> MIDLLQADGNALPSAVKLAYSPASKTFESYRVMTQVHTNDATKKVIVKLADTPQLTDVLNSTVQMPISVSWGGQVLSTTAKEFEAAALGYSASGVNGVSSSQELVISAAPKTAGTAPTAGNYSGVVSLVMTLGSDNKQVEKNITVTA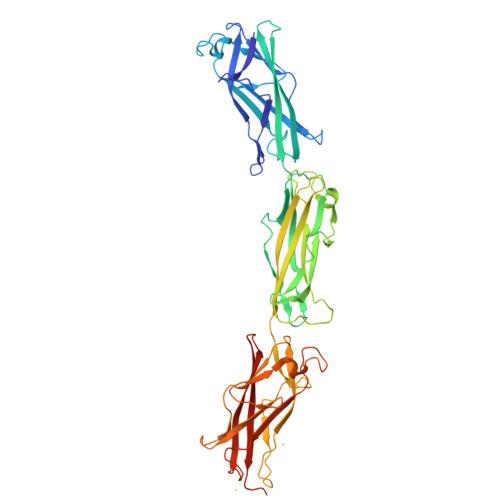SVDPVIDLLQADGNALPSAVKLAYSPASKTFESYRVMTQVHTNDATKKVIVKLADTPQLTDVLNSTVQMPISVSWGGQVLSTTAKEFEAAALGYSASGVNGVSSSQELVISAAPKTAGTAPTAGNYSGVVSLVMTLGSDNKQVEKNITVTASVDPVIDLLQADGNALPSAVKLAYSPASKTFESYRVMTQVHTNDATKKVIVKLADTPQLTDVLNSTVQMPISVSWGGQVLSTTAKEFEAAALGYSASGVNGVSSSQELVISAAPKTAGTAPTAGNYSGVVSLVMTLGSDNKQVEKNITVTASVDPVILEHHHHHH> MGSSHHHHHHSSGENLYFQGSHMTATATSAKAAAPACPRFDDPVHAAADPRVDVERITPDPVWRTTCGTLYRSDSRGPAVVFEQGFLPKDVIDGQYDIESYVLVAQPSPYVSTTYDHDLYKT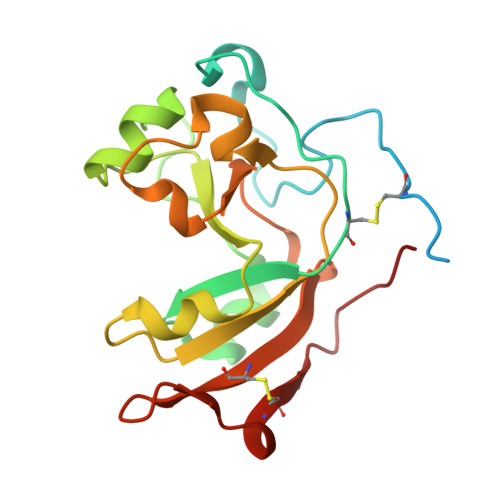WYKSGYNYYIDAPGGVDVNKTIGDRHKWADQVEVAFPGGIRTEFVIGVCPVDKKTRTEKMSECVGNPHYEPWH> GSGEVKMKLQEFVLN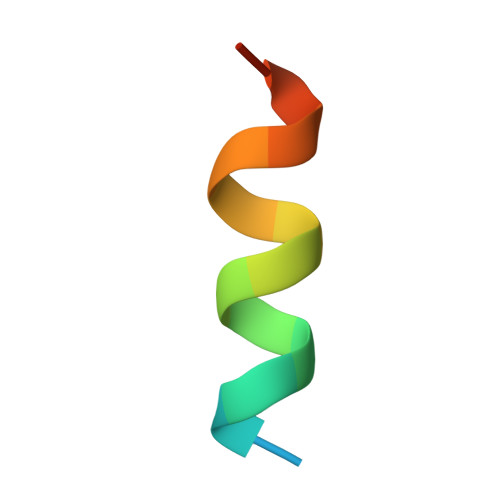KK Bdellovibrio bacteriovorus is a bacterium that preys upon a wide range of other Gram-negative bacteria, entering their periplasm and consuming them from within. Proteomic and structural analyses of vesicle contents reveal several fibre-like proteins, which we name the mosaic adhesive trimer (MAT) superfamily, and show localization on the predator surface before prey encounter. Structural studies reveal a variety of domain usages (and therefore binding capabilities) at the fibre C-termini, placing these on intertwined trimeric β-prisms. Using independent but complementary approaches, we identified and characterized a MAT superfamily of trimeric fibre proteins with diverse adhesive tips, able to fulfil the long-sought-after role of multiplicity of molecular recognition and handling of diverse epitopes (across a wide prey range), by the bacterial predator B. bacteriovorus.

We next determined the structure of Bd2740 (residues 517–626, 2.6 Å resolution), whose fold was previously cryptic. Our resulting structure reveals a variant of the C-type lectin fold, a widely dispersed superfamily named after its use of calcium to bind sugars, proteins and lipids. The fold has many structural homologues, the closest being snake venom agkisacucetin (PDB code 1v4l28, 2.1 Å RMSD). TopSearch22 analysis indicates that the majority of C-type lectins use a different face for trimerization, and the only homologue to match Bd2740 is the major viral adhesion protein Mtd from Bordetella bacteriophage (PDB code 2iou29), which binds host pertactin on its upper surface. The largest pockets and clefts are upwardly facing (distal to the fibre base) akin to Mtd. These observations reveal further potential for utilization of known adhesive folds at MAT fibre termini and show that these can diverge over time into distinct variants. We found that Bd2740–mCherry did locate to the CpoBBd0635-containing vesicle, deposited during predatory invasion, while Bd1334–mCherry and Bd2734–mCherry fluorescence were diffuse throughout the B. bacteriovorus cell. However, a slight reduction in prey entry efficiency was seen for deletion mutants of Bd2734 and Bd2740, which are structurally divergent but have similar expression profiles and are encoded at nearby genetic loci.

>HHHHHHASAPCDSGWTLINKGDPFCAKQQSVTGTNFATSMTQCLNNGGKLCDLQEAVGMCQTGFIPSNTTLWISQLADNSSAHVINCTSGSWSAGFYGFGVTVDGSNPILPYCCKGRR[3x]> MNDIVSAKVLEYKGKKLNFTPEDPAEETIPADELHEHLQKPSTARTKRLKERCRWKHASAGEFIEKSVTAGIERMRYLTEAHKASEGKPEAIRRALGLANVLNKSTLVLQEDEFIVGYHAEDPNMFPLYPELSHMAVQDYLRSDYSPQPADEAAAINEYWKPHSLQSKCQPYFDPADLGRMYQVSSMEAPSFASGYNSIVPPYETVLEDGLLARIKLAEKHIAEAQADMSTFPWNGTKGLDNIAKIDNWKAMVIACKAVISWARRQ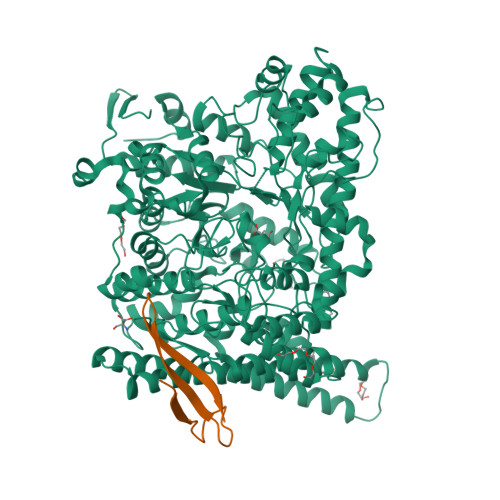GRLCKIVAENFETDPKRQAELLEIADICQRIPAEPCKGLKDAMQAKFFTFLICHAIERYASGYAQKEDTLLWPYYKASVVDKKFQPMSHMDAVELVEMERLKISEHGAGKSRAYREIFPGSNDLFILTVGGTNAKGEDACNDMTDAILEAAKRIRTAEPSIVFRYSKKNREKTLRWVFECIRDGLGYPSIKHDEIGTEQMKEYAKFSLNGNGATDEEAHNWVNVLCMSPGIHGRRKTQKTRSEGGGSIFPAKLLEISLNDGYDWSYADMQLGPKTGDLSSLKSFEDVWEAFRKQYQYAINLCISTKDVSRYFEQRFLQMPFVSAIDDGCMELGMDACALSEQPNGWHNPITTIVAANSLVAIKKLVFEEKKYTLEQLSQALKANWEGFEEMRVDFKRAPKWGNDDDYADGIITRFYEEIIGGEMRKITNYSGGPVMPTGQAVGLYMEVGSRTGPTPDGRFGGEAADDGGISPYMGTDKKGPTAVLRSVSKVQKNQKGNLLNQRLSVPIMRSKHGFEIWNSYIKTWHDLNIDHVQFNVVSTDEMRAAQREPEKHHDLIVRVSGYSARFVDIPTYGQNTIIARQEQDFSASDLEFLNVEISGTGSGSSHHHHHH;> MGTTTCKQCANFFPVPKDADDYEAGKADCVREKEDEKGKYWLSKPIFENSAQCEAFQTKR Wzc, an integral cytoplasmic membrane tyrosine autokinase protein serves as the master regulator of the biosynthesis and export of many bacterial capsular polysaccharides and exopolysaccharides. Wzc comprises a large periplasmic domain, two transmembrane helices and a C-terminal cytoplasmic kinase domain with a tyrosine-rich tail. Wzc regulates polymerisation functions through cycling the formation and dissociation of an octameric complex, driven by changes in the phosphorylation status of the tyrosine-rich tail. E. coli Wzc serves a model for a wider family of polysaccharide co-polymerases.

Here, we report the characterisation of the structures WzcK540M2YE (Y718E, Y717E), WzcK540M3YE (Y718E, Y717E and Y715E) and WzcK540M3YE_N711Y (an additional N711Y mutation) corresponding to different phosphorylation states. One intermediate, 2pY which has Y713 at the active site, does not follow the YxY pattern, since position 711 is asparagine. We show that it is binding of the i-2 tyrosine to the tyrosine pocket (where i is the number of the residue positioned at the kinase active site) orders the tail between the tyrosine at the active site and helix α23. A mutant of 2pY (Wzc3YE_N711Y) stabilises the C-terminal tail was functional in vivo, restoring immunoreactive CPS to levels approximating the wild type. This is consistent with a model in which the more stable the Wzc octamer the higher the Wzy activity. We note the reduction of CPS production by destabilising D28A and K701A mutants further support this model. The Wzc3YE_N711Y shows greater phosphorylation relative to Wzc3YE and proteomic analysis of purified WzcYF_713Y/N711Y reveals both N711Y and Y713 are phosphorylated. We propose that the YxY pattern serves as a molecular ratchet, that by selecting a tyrosine over phosphotyrosine, ensures phosphorylations in unidirectional (moving from the C to the N).

>[8x]MTSVTSKQSTILGSDEIDLGRVIGELIDHRKLIISITSVFTLFAILYALLATPIYETDALIQIEQKQGNAILSSLSQVLPDGQPQSAPETALLQSRMILGKTIDDLNLQIQIEQKYFPVIGRGLARLMGEKPGNIDITRLYLPDSDDISNNTPSIILTVKDKENYSINSDGIQLNGVVGTLLNEKGISLLVNEIDAKPGDQFVITQLPRLKAISDLLKSFSVADLGKDTGMLTLTLTGDNPKRISHILDSISQNYLAQNIARQAAQDAKSLEFLNQQLPKVRAELDSAEDKLNAYRKQKDSVDLNMEAKSVLDQIVNVDNQLNELTFREAEVSQLYTKEHPTYKALMEKRQTLQEEKSKLNKRVSSMPSTQQEVLRLSRDVESGRAVYLQLLNRQQELNIAKSSAIGNVRIIDNAVTDPNPVRPKKTIIIVIGVVLGLIVSVVLVLFQVFLRRGIESPEQLEEIGINVYASIPISEWLTKNARQSGKVRKNQSDTLLAVGNPADLAVEAIRGLRTSLHFAMMEAKNNVLMISGASPSAGMTFISSNLAATIAITGKKVLFIDADLRKGYAHKMFGHKNDKGLSEFLSGQAAAEMIIDKVEGGGFDYIGRGQIPPNPAELLMHPRFEQLLNWASQNYDLIIIDTPPILAVTDAAIIGRYAGTCLLVARFEKNTVKEIDVSMKRFEQSGVVVKGCILNGVVKKASSYYRYGHYHYGESEEDKKHHHHHH> MKPIEIHREQPAQHEAMIQLYLDPTLDWFRGHFPVQPLLPGVAQIDWVMHYAQTLLAPGWSFSSIEMVKFQFPLQPGNTLLLKINWDEKKHLLTFRYDLDTHNGSEGQTASQGKIKLCR;> MWSHPQFEKENLYFQGPDYLPVDRYLPVDRYLPHEAPMVLLEQVINVSDNHVHCQVTVSRDGVLSPFLNQDGHLPGWFAIEMMAQAIGVWSGWHRKERKEADSALGMLLGGRAVRCQVPAFTQGSVLD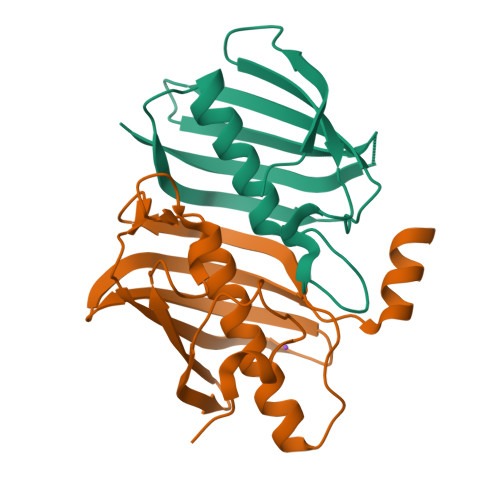IQMNLLLQDEKFGSFEGEISCYGTVLVTGRLNTYQPNKTELIQLINKQDGVA>[3x]MYRVFVFDLDGTLLNDNLEISEKDRRNIEKLSRKCYVVFASGRMLVSTLNVEKKYFKRTFPTIAYNGAIVYLPEEGVILNEKIPPEVAKDIIEYIKPLNVHWQAYIDDVLYSEKDNEEIKSYARHSNVDYRVEPNLSELVSKMGTTKLLLIDTPERLDELKEILSERFKDVVKVFKSFPTYLEIVPKNVDKGKALRFLRERMNWKKEEIV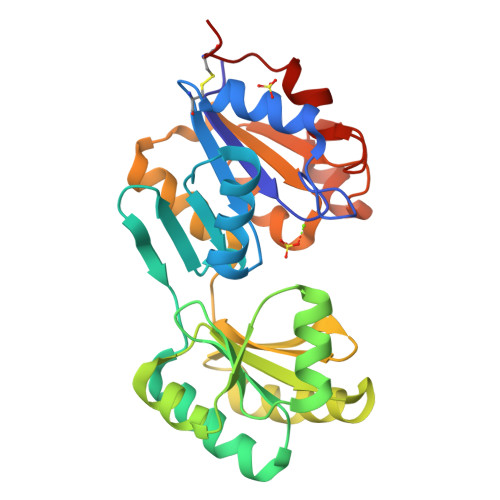VFGDNENDLFMFEEAGLRVAMENAIEKVKEASDIVTLTNNDSGVSYVLERISTDCLDE> GPLGSQELRLRVQGKEKHQMLEISLSPDSPLKVLMSH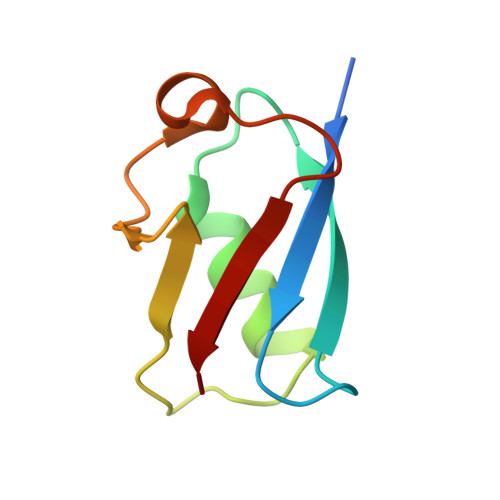YEEAMGLSGHKLSFFFDGTKLSGKELPADLGLESGDLIEVWG>MAITDILSAKDIESALSSCQAADSFNYKSFFSTVGLSSKTPDQIKKVFGILD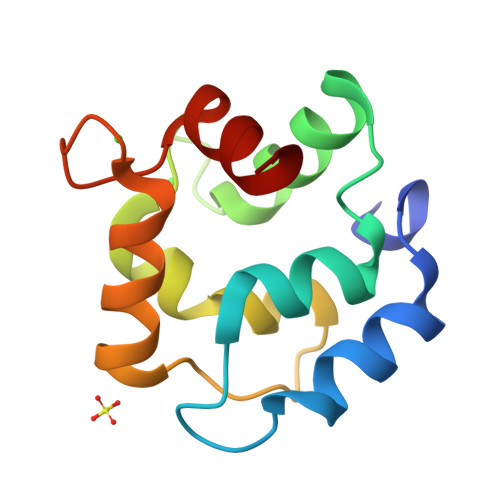QDKSGFIEEEELQLFLKNFSSSARVLTSAETKAFLAAGDTDGDGKIGVEEFQSLVKA[8x]>MRHPVVMGNWKLNGSKEMVVDLLNGLNAELEGVTGVDVAVAPPALFVDLAERTLTEAGSAIILGAQNT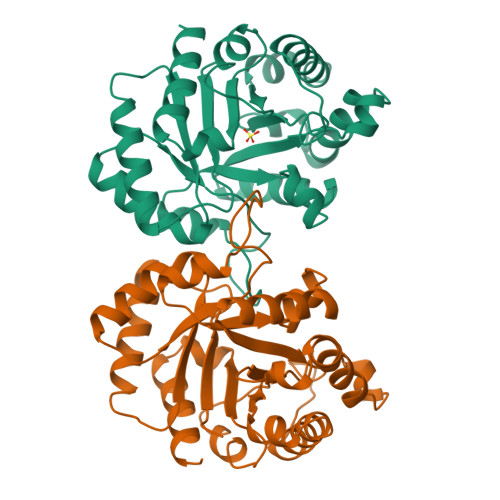DLNNSGAFTGDMSPAMLKEFGATHIIIGHSERREYHAESDEFVAKKFAFLKENGLTPVLCIGESDAQNEAGETMAVCARQLDAVINTQGVEALEGAIIAYEPIWAIGTGKAATAEDAQRIHAQIRAHIAEKSEAVAKNVVIQYGGSVKPENAAAYFAQPDIDGALVGGAALDAKSFAAIAKAAAEAKA[8x]> MVSKNKKLNLKDKYQYLTRDMAWEPTYQDKKDIFPEEDFEGIKITDWSQWEDPFRLTMDAYWKYQAEKEKKLYAIFDAFAQNNGHQNISDARYVNALKLFISGISPLEHAAFQGYSKVGRQFSGAGARVACQMQAIDELRHSQTQQHAMSHYNKHFNGLHDGPHMHDRVWYLSVPKSFFDDARSAGPFEFLTAISFSFEYVLTNLLFVPFMSGAAYNGD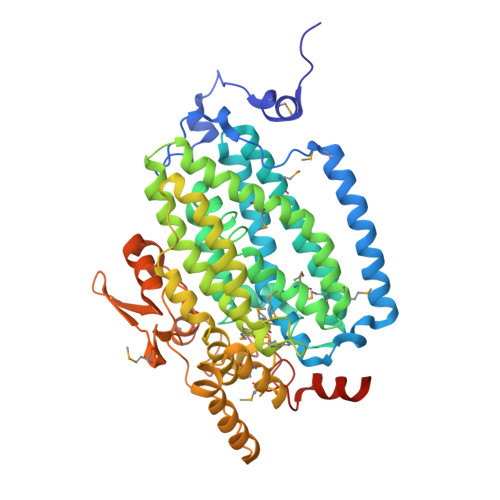MATVTFGFSAQSDEARHMTLGLEVIKFILEQHEDNVPIVQRWIDKWFWRGFRLLSLVSMMMDYMLPNKVMSWSEAWEVYYEQNGGALFKDLERYGIRPPKYQDVANDAKHHLSHQLWTTFYQYCQATNFHTWIPEKEEMDWMSEKYPDTFDKYYRPRYEYLAKEAAAGRRFYNNTLPQLCQVCQIPTIFTEKDAPTMLSHRQIEHEGERYHFCSDGCCDIFKHEPEKYIQAWLPVHQIYQGNCEGGDLETVVQKYYHINIGEDNFDYVGSPDQKHWLSIKGRKPADKNQDDA> PISPIETVPVKLKPGMDGPKVKQWPLTEEKIKALVEICTEMEKEGKISKIGPENPYNTPVFAIKKKDSTKWRKLVDFRELNKRTQDFWEVQLGIPHPAGLKKKKSVTVLDVGDAYFSVPLDEDFRKYTAFTIPSINNETPGIRYQYNVLPQGWKGSPAIFQSSMTKILEPFRKQNPDIVICQYMDDLYVG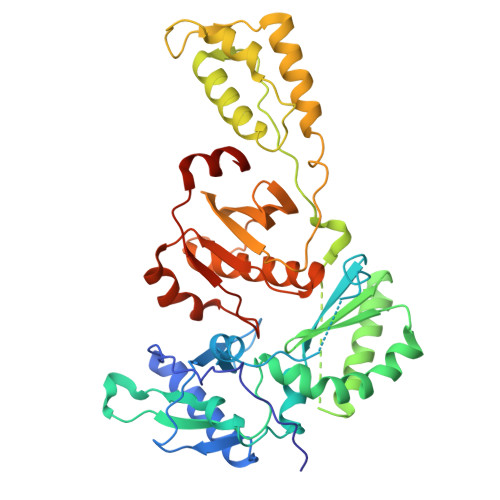SDLEIGQHRTKIEELRQHLLRWGLTTPDKKHQKEPPFLWMGYELHPDKWTVQPIVLPEKDSWTVNDIQKLVGKLNWASQIYPGIKVRQLCKLLRGTKALTEVIPLTEEAELELAENREILKEPVHGVYYDPSKDLIAEIQKQGQGQWTYQIYQEPFKNLKTGKYARMRGAHTNDVKQLTEAVQKITTESIVIWGKTPKFKLPIQKETWETWWTEYWQATWIPEWEFVNTPPLVKLWYQLEKEPIVGAETF> MMRGSHHHHHTDPISYIIRKADSVNKALDSAVPLREPLKIHEAMRYSLLAGGKRV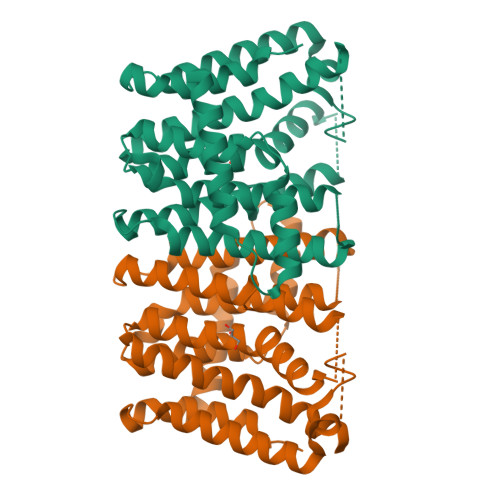RPVLCIAACELVGGEESLAMPAACAVEMIHTMSLIHDDVYGEDVAVLAGDALLSFAFEHLASATSSEVSPARVVRAVGELAKAIGTEGLVAGQVVDISNVGLEHLKFIHLHKTAALLEASAVLGGIIGGGSDEEIERLRKFARCIGLLFQVVDDILDVTIADKLTYPKLMGLEKSREFAEKLNTEARDQLLGFDSDKVAPLLALANYIANRQN MALONALDEHYDE | C3 H4 O2 | 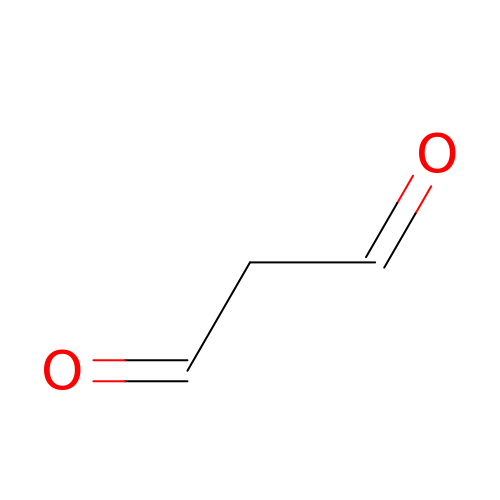WSMYVTOQOOLQHP-UHFFFAOYSA-N> MEEVVLITVPSALVAVKIAHALVEERLAACVNIVPGLTSIYREEGSVVSDHELLLLVKTTTDAFPKLKERVKE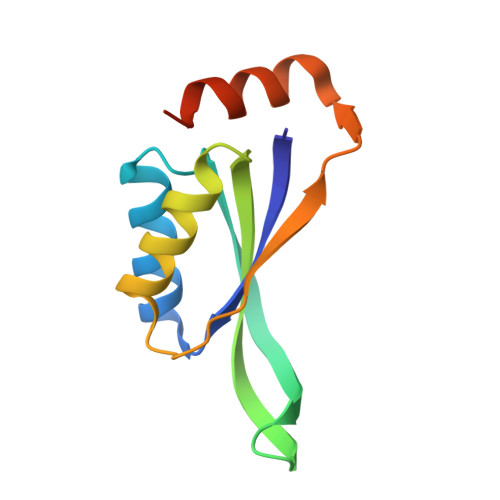LHPYEVPEIVALPIAEGNREYLDWLRENTGLEHHHHHH>[2x]SHMENSGGNAFVPAGNQQEAHWTINLKDADIREFIDQISEITGETFVVDPRVKGQVSVVSKAQLSLSEVYQLFLSVMSTHGFTVVAQGDQARIVPNAEAKTE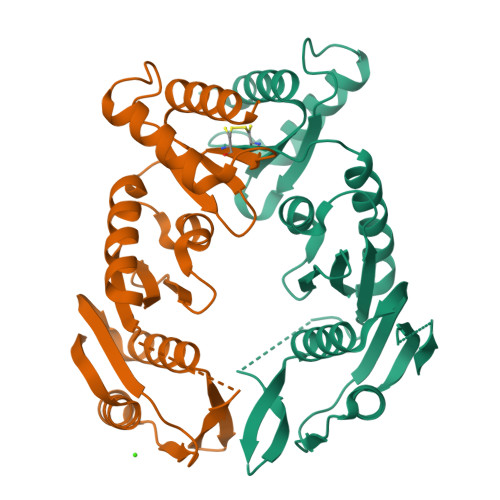AGGGQSAPDRLETRVIQVQQSPVSELIPLIRPLVPQYGHLAAVPSANALIISDRSANIARIEDVIRQLDQKGSHDYCVINLRYGWVMDAAEVLNNAMSRGQAKGAAGAQVIADARTNRLIILGPPQARAKLVQLAQSLDTPTAR> GLPSLCYEPADSGSGTKSEKRIYYNSARKQCLRFTYNGKGGNANNFIHTFDCQ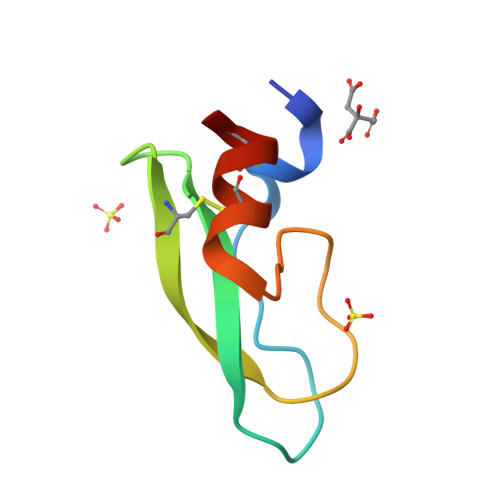HTCLYK> HM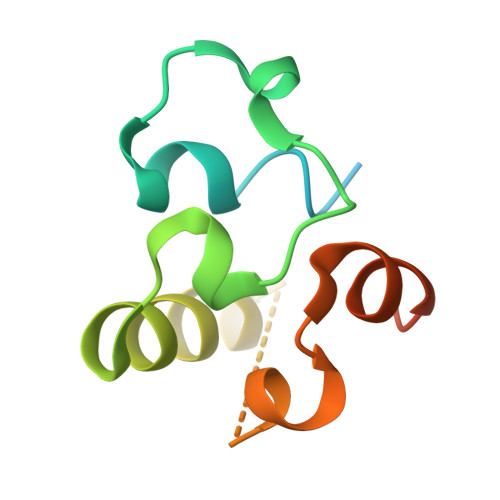PREPVTPDSDHPDPVETVRQLTAHVLGLTAAADVEMTRSFKDLGFDSLMSVELRDRLCAATGLSLATTLLYDHPSPAETAEFVRARLTGDEA>SMPNHQKVVLVGDGAVGSSYAFAMAQQGIAEEFVIVDVVKDRTKGDALDLEDAQAFTAPKKIYSGEYSDCKDADLVVITAGAPQKPGESRLDLVNKNLNILSSIVKPVVDSGFDGIFLVAANPVDILTYATWKFSGFPKERVIGSGTSLDSSRLRVALGKQFNVDPRSVDAYIMGEHGDSEFAAYSTATIGTRPVRDVAKEQGVSDDDLAKLEDGVRNKAYDIINLKGATFYGIGTALMRISKAILRDENAVLPVGAYMDGQYGLNDIYIGTPAIIGGTG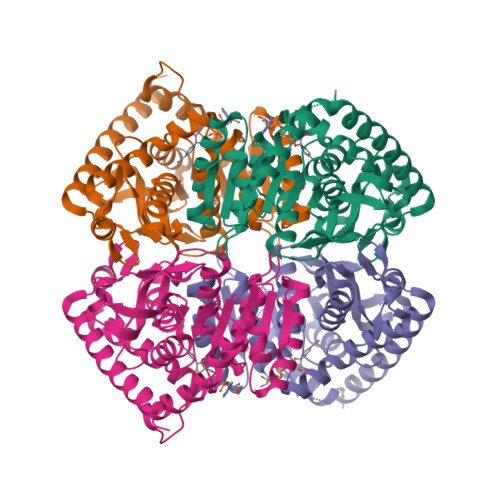LKQIIESPLSADELKKMQDSAATLKKVLNDGLAELENK[4x]We discovered that the archaeal PAC1-PAC2 homolog PbaB functions as an ATP-independent proteasome activator. We revealed that binding of PbaB to the 20S proteasome depended on its C-terminal HbYX motif. Moreover, we revealed that PbaB activates the proteasome irrespective of the presence of ATP. Analytical ultracentrifugation also confirmed that PbaB forms a stable homotetramer in solution.

Using the Au3+-bound crystal belonging to space group C2221 with four molecules per asymmetric unit, the atomic coordinates were determined by the single-wavelength anomalous dispersion (SAD) method. The crystal structure of PbaB exhibited a tetrameric structure with a remarkably large (1227 Å2) surface area buried through quaternary structure formation. Each PbaB protomer has a single domain comprised of a central mixed β-sheet (β1–β3–β6–β7–β2–β8–β12–β9–β10) flanked by four α-helices (α1, α3, α5, and α6) on one side and one β-strand (β11) and two α-helices (α2 and α4) on the other side, thereby making an overall three-layered αβα fold. Extended β-hairpin (β4–β5) is involved in tetramerization by forming a three-stranded anti-parallel β-sheet with β11 from the adjoining molecule. In the tetramer structure, the C-terminal α-helices (α6) are located peripheral to the core domain and extend in the same direction, yielding a tentacle-like structure. The α6 helices showed poor electron densities with high crystallographic B values (45–100 Å2), suggesting that the C-terminal segments had flexible properties. Intriguingly, PbaB accelerated proteasomal degradation of LFP and α-synuclein by about 3- and 2.5-fold, respectively, whereas the mutated PbaB that lacked the C-terminal HbYX motif (Gly-Tyr-Leu) did not accelerate proteasomal degradation. Truncation of the eight residues of the C-terminus significantly compromised chaperone activity, and deletion of the α6 helix markedly impaired the suppression of aggregation of citrate synthase. These findings indicated that the tentacle-like C-terminal segments of the PbaB tetramer are critically involved in capturing unfolded proteins. Based on the electron tomography and biochemical data, we hypothesize that a subset of C-terminal segments function as gate openers to activate the 20S proteasome, and the remaining unanchored C-terminal segments are involved in capturing proteasomal substrates.

>[4x]GSHMEEGGTRNREEGKMKETTIVVYERPDIYDPIFIEGLPGIGLVGKLAAEHLIQELKAKKFAELYSPHFMHQVLIRKNSVVELMKNEFYYWKSPDDEHRDLIIVTGDTQVPPTDSYGHFEVAGKMLDFVQEFGTREIITMGGYQVPEIQGEPRVLAAVTHEDLIEYYKSKLEGCSVEVIWREDEGGAIVGAAGLLLGIGKLRGMFGISLLGESLGYIVDAKAAKAVLSAVTKILGLEIDMTALDERAKETEEILRKVEEMQRAMMEQVTPKLPHEEEDRGYL> ENLYFQGASLTEIEHLVQSVCKSYRETCQLRLEDLLRQRSNIFSREEVTGYQRKSMWEMWERCAHHLTEAIQYVVEFAKRLSGFMELCQNDQIVLLKAGAMEVVLVRMCRAYNADNRTVFFEGKYGGMELFRALGCSELISSIFDFSHSLSALHFSEDEIALYTALVLINAHRPGLQEKRKVEQLQYNLELAFHHHLCKTHRQSILAKLPPKGKLRSLCSQHVERLQIFQHLHPIVVQAAFPP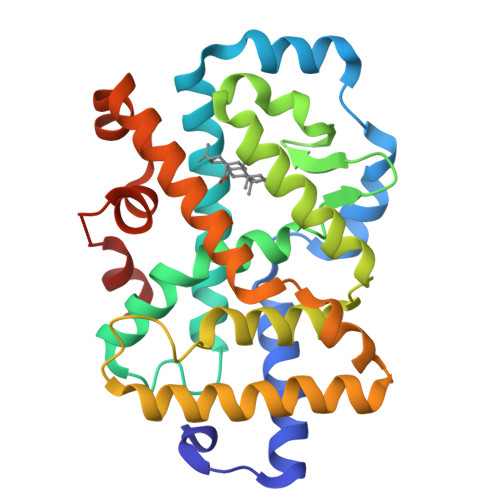LYKELFSGGSGKEKHKILHRLLQDSS> MATSELSSEVSEENSERREAFWAEWKDLTLSTRPEE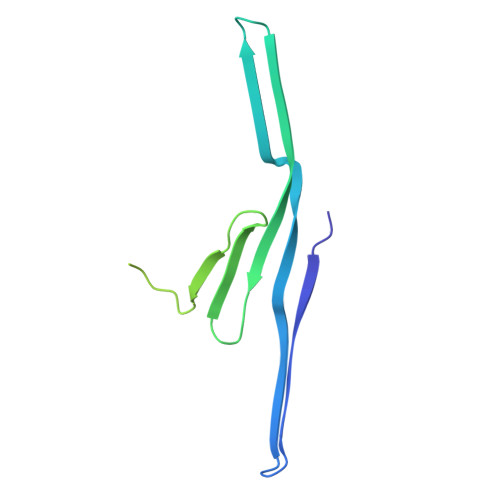GSSLHEEDTQRHETYHQQGQSQVLVQRSPWLMMRMGILGRGLQEYQLPYQRVLPLPIFTPAKMGATKEEREDTPIQLQELLALETALGGQSVDRQEVAEITKQLPPVVPVSKPGALRRSLSRSMSQEAQRG> MGEDVIDSLQLNELLNAGEYKIGELTFQSIRSSQELQKKNTIVNLFGIVKDFTPSRQSLHGTKDWVTTVYLWDPTCDTSSIGLQIHLFSKQGNDLPV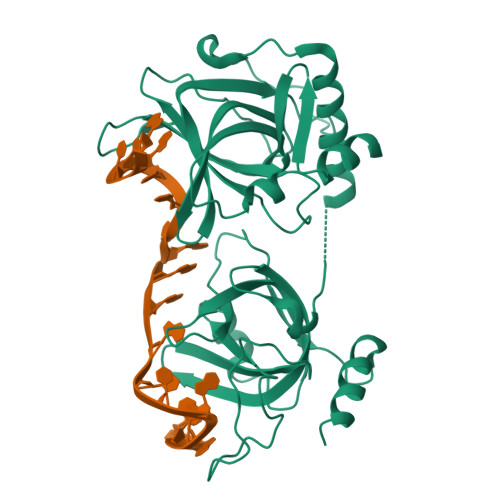IKQVGQPLLLHQITLRSYRDRTQGLSKDQFRYALWPDFSSNSKDTLCPQPMPRLMKTGDKEEQFALLLNKIWDEQTNKHKNGELLSTSSARQNQTGLSYPSVSFSLLSQITPHQRCSFYAQVIKTWYSDKNFTLYVTDYTENELFFPMSPYTSSSRWRGPFGRFSIRCILWDEHDFYCRNYIKEGDYVVMKNVRTKIDHLGYLECILHGDSAKRYNMSIEKVDSEEPELNEIKSRKRLYVQN> MSDTMVVNGSGGVPAFLFSGSTLSSYRPNFEANSIT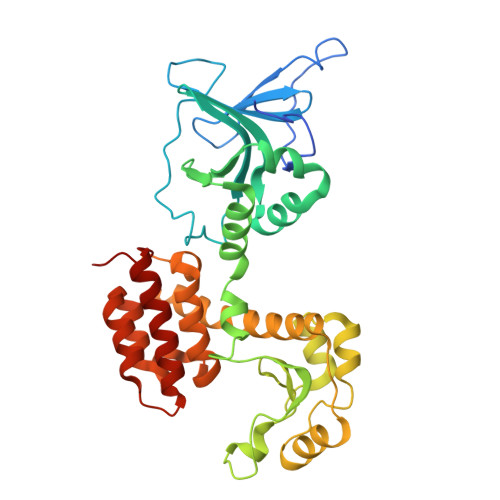IALPHYVDLPGRSNFKLMYIMGFPIDTEMEKDSEYSNKIRQESKISKTEGTVSYEQKITVETGQEKDGVKVYRVMVLEGTIAESIEHLDKKENEDILNNNRNRIVLADNTVINFDNISQLKEFLRRSVNIVDHDIFSSNGFEGFNPTSHFPSNPSSDYFNSTGVAFGSGVDLGQRSKQDLLNDGVPQYIADRLDGYYMLRGKEAYDKVRTAPLTLSDNEAHLLSNIYIDKFSHKIEGLFNDANIGLRFSDLPLRTRTALVSIGYQKGFKLSRTAPTVWNKVIAKDWNGLVNAFNNIVDGMSDRRKREGALVQKDIDSGLLKLE>MTIPTLYMNDGMNAQSSQALHIQTYCNSVRQQIPVDFGRFPNLRESERQINTGLGAARQHAEHYLKDIQPLIIRNVTNIQDYFETQNLISTVMPSGATKEQWLSALGMVSDKAKEYQEVSANTRRTIGSLNDKLIIDSNNYQLIVVNLNNVVNGNNGVLEQLNRDIDGINAAIDGAIAGIVVGGLLVIGGAIVTAIGAVAGLVTAGTSTPVVMGGIAMMTAGAGGVIGGAIVLDKSLSAREKLYRDRSQLNSEVLVASQIGSGYRGLQTQAQSAVTAATQMNNAWDSLTSELETLNANLRKGIIDDSFLRQLFLTASQTSVTKVLDGTKIIKQQMAGVVVREVPANQSIADFVK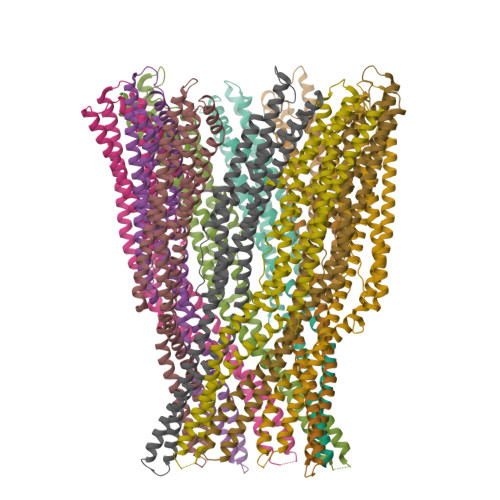RLAALEHHHHHH[10x]> SVTIDH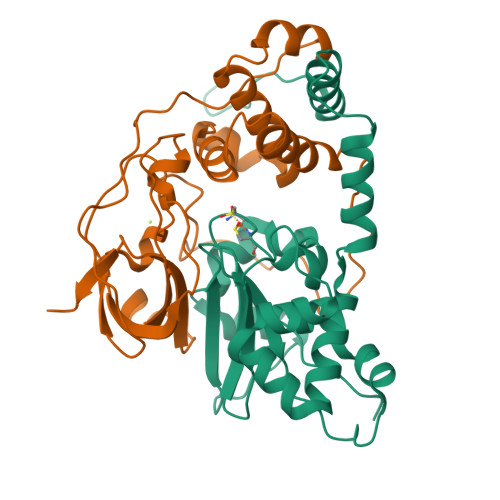TTENAAPAQAPVSDRAWALFRALDGKGLVPDGYVEGWKKTFEEDFSPRRGAELVARAWTDPEFRQLLLTDGTAAVAQYGYLGPNGEYIVAVEDTPTLKNVIVCSLCSCTAWPILGLPPTWYKSFEYRARVVREPRKVLSEMGTEIASDIEIRVYDTTAETRYMVLPQRPAGTEGWSQEQLQEIVTKDCLIGVAIPQVPTV;> MDGVHDLAGVQGFGKVPHTVNADIGPTFHAEWEHLPYSLMFAGVAELGAFSVDEVRYVVERMEPRHYMMTPYYERYVIGVATLMVEKGILTQDELESLAGGPFPLSRPSESEGRPAPVETTTFEVGQRVRVRDEYVPGHIRMPAYCRGRVGTISHRTTEKWPFPDAIGHGRNDAGEEPTYHVKFAAEELFGSDTDGGSVVVDLFEGYLEPAA> SNAMPYTWKFLGISKQLSLENGIAKLNQLLNLEVDLDIQTIRVPSDPDGGTAADEYIRYEMRLDISNLDEGTYSKFIFLGNSKMEVPMFLCYCGTDNRNEVVLQWLKAEYGVIMWPIKFEQKTMIKLADASIVHVTKENIEQITWFSSKLYFEPETQDKNLRQFSIEIPRESCE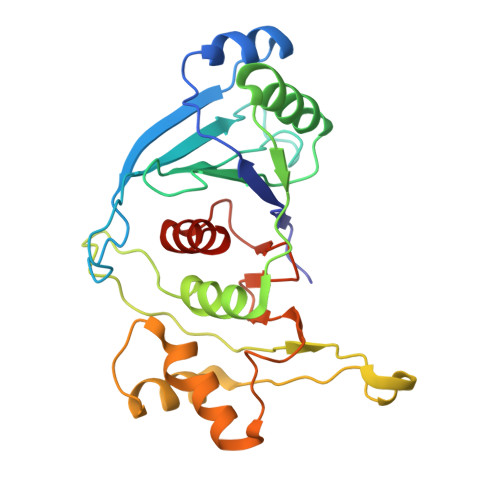GLALGYGNTMHPYNDAIVPYIYNETGMAVERLPLTSVILAGHTKIMRESIVTSTRSLRNRVLAVVLQSIQFTSE1-{3-[3-{[2-(4-fluoropiperidin-1-yl)ethyl]sulfanyl}-4-(trifluoromethyl)phenyl]-1-[(2S)-2-hydroxy-3-(piperidin-1-yl)propyl]-1,4,6,7-tetrahydro-5H-pyrazolo[4,3-c]pyridin-5-yl}-2-hydroxyethan-1-one 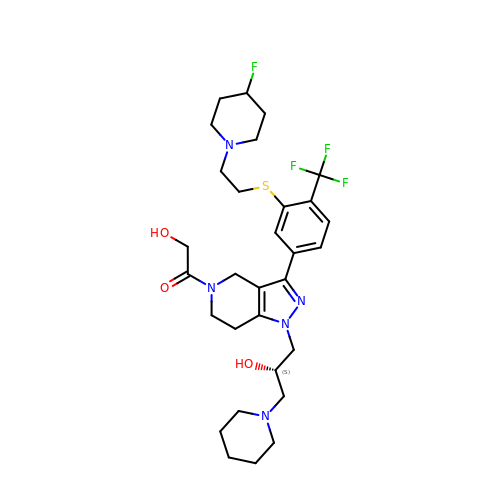| C30 H41 F4 N5 O3 S | QFMAXTIVGRIBEI-QHCPKHFHSA-N8-(1-benzothiophen-5-yl)-7-[(4-chlorophenyl)methyl]-6-{[(1R)-1-cyclopropylethyl]amino}-7H-purine-2-carboxylic 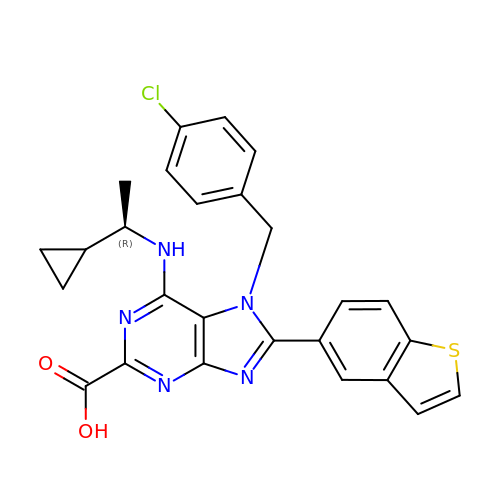acid | C26 H22 Cl N5 O2 S | VYDVBUHEXZQWED-CQSZACIVSA-N6-ethoxy-1,3-benzothiazole-2-sulfonamide | C9 H10 N2 O3 S2 | 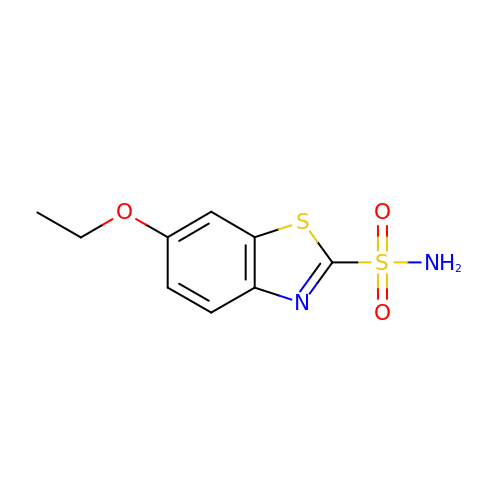OUZWUKMCLIBBOG-UHFFFAOYSA-N> GGGASEFVDMACWPQLRLLLWKNLTFRRRQTCQLLLEVAWPLFIFLILISVRLSYPPYEQHECHFPNKAMPSAGTLPWVQGIICNANNPCFRYPTPGEAPGVVGNFNKSIVARLFSDARRLLLYSQKDTSMKDMRKVLRTLQQIKKSSSNLKLQDFLVDNETFSGFLYHNLSLPKSTVDKMLRADVILHKVFLQGYQLHLTSLCNGSKSEEMIQLGDQEVSELCGLPREKLAAAERVLRSNMDILKPILRTLNSTSPFPSKELAEATKTLLHSLGTLAQELFSMRSWSDMRQEVMFLTNVNSSSSSTQIYQAVSRIVCGHPEGGGLKIKSLNWYEDNNYKALFGGNGTEEDAETFYDNSTTPYCNDLMKNLESSPLSRIIWKALKPLLVGKILYTPDTPATRQVMAEVNKTFQELAVFHDLEGMWEELSPKIWTFMENSQEMDLVRMLLDSRDNDHFWEQQLDGLDWTAQDIVAFLAKHPEDVQSSNGSVYTWREAFNETNQAIRTISRFMECVNLNKLEPIATEVWLINKSMELLDERKFWAGIVFTGITPGSIELPHHVKYKIRMDIDNVERTNKIKDGYWDPGPRADPFEDMRYVWGGFA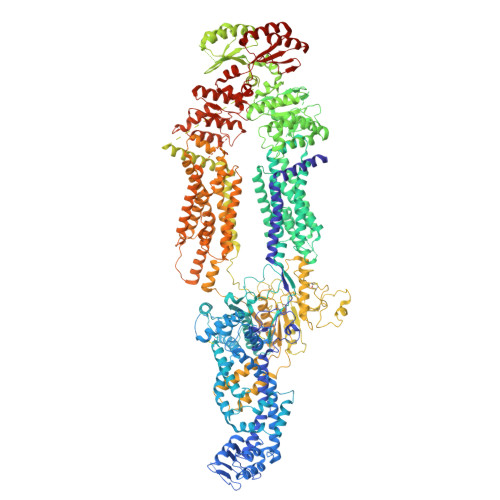YLQDVVEQAIIRVLTGTEKKTGVYMQQMPYPCYVDDIFLRVMSRSMPLFMTLAWIYSVAVIIKGIVYEKEARLKETMRIMGLDNSILWFSWFISSLIPLLVSAGLLVVILKLGNLLPYSDPSVVFVFLSVFAVVTILQCFLISTLFSRANLAAACGGIIYFTLYLPYVLCVAWQDYVGFTLKIFASLLSPVAFGFGCEYFALFEEQGIGVQWDNLFESPVEEDGFNLTTSVSMMLFDTFLYGVMTWYIEAVFPGQYGIPRPWYFPCTKSYWFGEESDEKSHPGSNQKRISEICMEEEPTHLKLGVSIQNLVKVYRDGMKVAVDGLALNFYEGQITSFLGHNGAGKTTTMSILTGLFPPTSGTAYILGKDIRSEMSTIRQNLGVCPQHNVLFDMLTVEEHIWFYARLKGLSEKHVKAEMEQMALDVGLPSSKLKSKTSQLSGGMQRKLSVALAFVGGSKVVILDEPTAGVDPYSRRGIWELLLKYRQGRTIILSTHHMDEADVLGDRIAIISHGKLCCVGSSLFLKNQLGTGYYLTLVKKDVESSLSSCRNSSSTVSYLKKEDSVSQSSSDAGLGSDHESDTLTIDVSAISNLIRKHVSEARLVEDIGHELTYVLPYEAAKEGAFVELFHEIDDRLSDLGISSYGISETTLEEIFLKVAEESGVDAETSDGTLPARRNRRAFGDKQSCLRPFTEDDAADPNDSDIDPESRETDLLSGMDGKGSYQVKGWKLTQQQFVALLWKRLLIARRSRKGFFAQIVLPAVFVCIALVFSLIVPPFGKYPSLELQPWMYNEQYTFVSNDAPEDTGTLELLNALTKDPGFGTRCMEGNPIPDTPCQAGEEEWTTAPVPQTIMDLFQNGNWTMQNPSPACQCSSDKIKKMLPVCPPGAGGLPPPQRKQNTADILQDLTGRNISDYLVKTYVQIIAKSLKNKIWVNEFRYGGFSLGVSNTQALPPSQEVNDAIKQMKKHLKLAKDSSADRFLNSLGRFMTGLDTKNNVKVWFNNKGWHAISSFLNVINNAILRANLQKGENPSHYGITAFNHPLNLTKQQLSEVALMTTSVDVLVSICVIFAMSFVPASFVVFLIQERVSKAKHLQFISGVKPVIYWLSNFVWDMCNYVVPATLVIIIFICFQQKSYVSSTNLPVLALLLLLYGWSITPLMYPASFVFKIPSTAYVVLTSVNLFIGINGSVATFVLELFTDNKLNNINDILKSVFLIFPHFCLGRGLIDMVKNQAMADALERFGENRFVSPLSWDLVGRNLFAMAVEGVVFFLITVLIQYRFFIRPRPVNAKLSPLNDEDEDVRRERQRILDGGGQNDILEIKELTKIYRRKRKPAVDRICVGIPPGECFGLLGVNGAGKSSTFKMLTGDTTVTRGDAFLNKNSILSNIHEVHQNMGYCPQFDAITELLTGREHVEFFALLRGVPEKEVGKVGEWAIRKLGLVKYGEKYAGNYSGGNKRKLSTAMALIGGPPVVFLDEPTTGMDPKARRFLWNCALSVVKEGRSVVLTSHSMEECEALCTRMAIMVNGRFRCLGSVQHLKNRFGDGYTIVVRIAGSNPDLKPVQDFFGLAFPGSVLKEKHRNMLQYQLPSSLSSLARIFSILSQSKKRLHIEDYSVSQTTLDQVFVNFAKDQSDDDHLKDLSLHKNQTVVDVAVLTSFLQDEKVKESYV> SNAADQLRTRGEAANDIRSKKVLIIGAGSLGSMIAENLMRIGVVSQGILDADLLQTGNLSRHALTMTSVGHNKAAALVEHLNRILPDASARSFSCAFPPESEVAKNSLRQYDVIIDCTGDDGVLK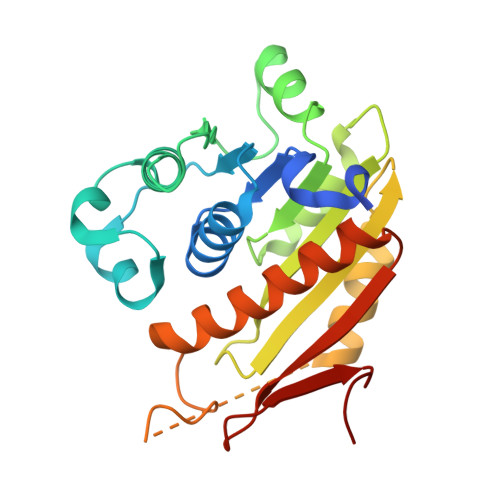SLAAFDWKSEKIFISLAMTWRAEGLFAFAASETSFPVTDASSRFNASASPEIDMDEARIEGIGAWHPVFPARADDVQLWAAVGTKFICRVVSAPGRIYEYFKQMPDGTVEKEPHEYGSG>[4x]MKEKLVAIVGPTAVGKTKTSVMLAKRLNGEVISGDSMQVYRGMDIGTAKITAEEMDGVPHHLIDIKDPSESFSVADFQDLATPLITEIHERGRLPFLVGGTGLYVNAVIHQFNLGDIRADEDYRHELEAFVNSYGVQA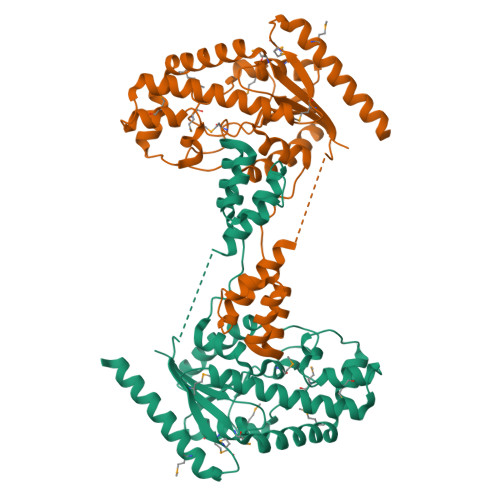LHDKLSKIDPKAAAAIHPNNYRRVIRALEIIKLTGKTVTEQARHEEETPSPYNLVMIGLTMERDVLYDRINRRVDQMVEEGLIDEAKKLYDRGIRDCQSVQAIGYKEMYDYLDGNVTLEEAIDTLKRNSRRYAKRQLTWFRNKANVTWFDMTDVDFDKKIMEIHNFIAGKLEEKSKLEHHHHHH>[6x]MSSLSRELVFLILQFLDEEKFKETVHKLEQESGFFFNMKYFEEKVHAGEWDEVEKYLSGFTKVDDNRYSMKIFFEIRKQKYLEALDRHDRAKAVDILVKDLKVFSTFNEELYKEITQLLTL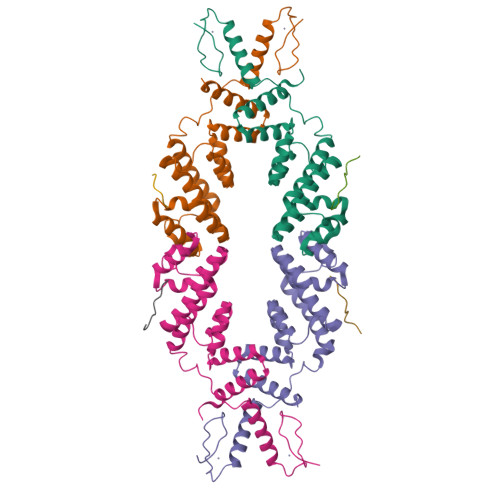ENFRENEQLSKYGDTKSARSIMLIELKKLIEANPLFREKLVFPTLKASRLRTLINQSLNWQHQLCKNPRPNPDIKTLFTDHTCTPPNG;>[6x]SETELDLALGL>MLTRIHGGRVVDPTAGRDAVGDVWIEDGRVVAPSERAPDQTIDATGCVVMAGGVEVHSHIAGGNVVMSRLLLPDLYVSESAPNGHPFAHAGGSGSWIGANYARMGYTTAVEPALPPSNALATHLELADIPLLDRGGLAVLGNDDHLLQLLRDGEGKQAVRDLVQQTLAHSRGLGVKCINAGGASAFKDGVLKLSLDDEIPCYGLSTRKIMSALLDAVEEIGVPHPLHVHCNNLGLPGADDSLVATLEAAEGRRIHFAHAQFYAYGVVDPENPMTGGFRSAAERINAAMEAHPNATYDVGQVVFGQTVTISLDILRQFGGRKGAKPKKWVISAGDAEGGGVVPFLYRPRGPVSSLQWAIGLELMLLSSNPERTILTTDHPNGGVFTEYPRIIHLLMDAEERAKEIATLPAIVGERSGLPKIEREYSFSEIAQLTRSGPAKLLGLTDRGHLREGAKADVAIYRDDTDRTAMFSRAKLVLKDGQPIVEDGEVVAWFSGKTLSLNVEADAGMEKRAESYLQDRFGAGLDTFAVPDAAFPENTGTFEDVACRA[4x];>[4x]AAWVKGGAADVDAAVEAAADL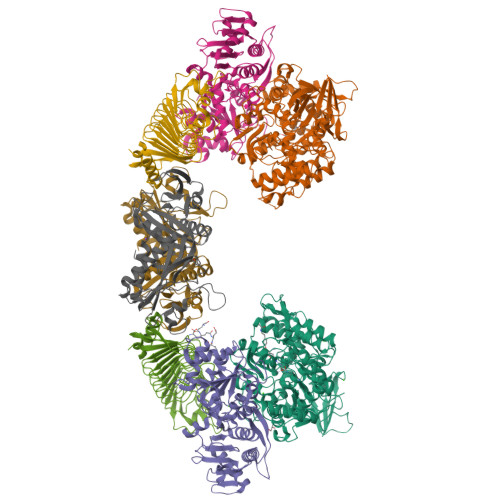LAASRVPVLAGLSAEVSALRAAYRLAETLGASLDPVSGPSVYAELGALSAGGAMSTTRAETIGRADVILIVGNRPWDGELIAEIAAAAPSRGRAAGAERALLSLGGPQNGAIRHVAYAADAGGLTISLGHLRAFAKGHLAGEAAFADLAKRLFAAQYGVIVYDPEEVGELGAEMLQGLIRDLNESTRFFALTLADPFQGRAAVQLSAWTTGQAPRVGFGRHQPEHDSWRFDSARQIAAGEADAALWLASLPAPRPAWLGSLPTIAIVGEGSQEAAGETAEVVITVGVPGQSVGGALWNDRRGVIAYAEASDPAKTPAETETAAGVLTRIRDRLIEKGVSC;>[4x]STLRLRGDLPERVDLLNITPLALSGLSETEAGKLAIGTSRRGLTLGDVFEIRLDGSDSLVIEGGSARLDRVGAALSQGSIRVEGDVGQRLGEGMAAGTLTVTGSAGPYAGTGATGGTITIEGDAGDHAGGAVYAAKAGLDGATLVIKGAAGDHLGDRMRRGMILAGSAGAFAASRMIAGTIVVSGALGDHPGYGMRRGTLIAGSHGTLLPTFVETGTPDLVFVRLLAQSLKHLGAAQANLLSGTLRRYSGDLATLGKGELFVPAHGSAWSHPQFEK;>SDFTLNGIKVEDTFAEAFDVAGTAIIVTNDTPKWAMIAATVMTGFATSVIGCGAEAGIDAELSPDETPDGRPGVRILLFGFEPNGLKDQLLKRVGQCILTCPGTACFAGVEGPTKIKLGGAIRYFGDGFAVAKRLPDHEGKMRRYWRIPVMDGEFLCEDSVRAVDGAVGGGNLLFLGRKHADTLIVAEIAVEAAKAIPGAILPFPGGIVRSGSKVGGRTKGMMASTNDAYCPTLKGRAGSALPPECGVVLEIVIDALTSAAVAESMRAALHAATEIGAQHGLVAVTAGNYGGNLGRHHYHLRDLLEKPAA[4x]GP4, a new Ralstonia solanacearum phage, is a short-tailed phage. The GP4 head contains 540 copies of major capsid protein (MCP) gp2 and 540 copies of cement protein (CP) gp1 arranged in an icosahedral shell with a triangulation number T = 9. The structures of gp2 and gp1 show a canonical HK97-like fold and an Ig-like fold, respectively. The trimeric CPs stick on the surface of the head along the quasi-threefold axis of the icosahedron generating a sandwiched three-layer electrostatic complementary potential, thereby enhancing the head stability.

Finally, we obtained a 3.7 Å resolution density map of the GP4 head that allowed us to build the full atomic models of the MCPs and CPs in the asymmetric unit of the icosahedron. Therefore, the asymmetric unit of the icosahedron contains 9 monomers of gp2, which include one E-hexon, one-third C-hexon, and one-fifth penton and the 9 monomers of gp1. According to the gp5 domain nomenclature in HK97, each gp2 monomer can be divided into four domains: an especially extended N-arm domain (residues 2–47), a long β-hairpin E-loop domain (residues 48–91), a P-domain (residues 92–140 and 307–342) containing two α-helices and a three-stranded β-sheet, and a highly complex A-domain (residues 141–307 and 343–367) including the long C-arm (residues 348–367). The superposition of the nine monomers (named A-I) of gp2 in the asymmetric unit of the head shows significant conformational changes in the N-arms and E-loops resulting in large-scale swinging. The helix α5 (residues 245–255) of monomer A (from penton) adopts a drastically different conformation to the other eight monomers, which results in a greater curvature in the central conformations of the pentons than in the hexons. Accompanying the movements of the α5 helices, the five bulky sidechains (Trp245) in the penton point to the central pore and form a hydrophobic core. In contrast, the sidechain Trp245 in the hexon flips to the opposite direction and inserts into a hydrophobic pocket formed by Leu237, Leu246, Pro261, Ile262, and Leu267 in the same MCP monomer. The structure of the nine CP monomers (named J-R) in the asymmetric unit are basically identical, which is also true of the nine CPs of KHP30. Three acid residues (Asp23) in the trimeric CP point to the axial center of the trimer and are located on the lower surface of the trimer, separated by a distance of approximately 3Å. In addition, along each quasi-three-fold axis, a three-layered sandwich interface structure is formed by complex electrostatic interactions to maintain the stability of the quasi-three-fold axis.

>MSSTVIAFGDPKAQKKWSSELAVDIRKKSYFESRFIGTSENAVIQRKTEVESDAGDRVSFDLSVRLRGQPTFGDDRVEGKEENLKFYTDEVIIDQVRHSVSAGGRMSRKRTAHDLRKTGRDRLGDYFYQLTDELFFMYLSGARGINKDFILPTSFTGYAKNPFNTPDAAHLLYGGVATSKASLANTDTMSRVVIERANVQATMMQAQDPETANMVPVSVEGEDRYVCVMSPFQEHSLRTSDAAGWLEIQKAAAAAEGRNNPIFKGGLGMIGNTVLHSHRNVVRFSDYGAGSDQPAARALFMGRQAAVVAYGTKGGLRYDWQEETKDYGNEPTVASGFIAGIKKTRFNDRDFGVISIDTYAKDPNPNNPA[9x];>[9x]MALIQSDFAQGIRMTPVPDCAGDVTACRFDITLKNAPAAGDIIELGVLPGNAVPVEAILDVDDLDTGGAPTITLDVGIMSGPVGKNDPARTCGNELFAASTVGQAGGVVRATASSAFRIQKAEDHRSVGVKVAAGPATGAAGKTIALILFYVQGTSQ>[2x]MSLKTVAVIGAMEQEIELLREMMENVKAVSFGRFSAYEGELAGKRMVLA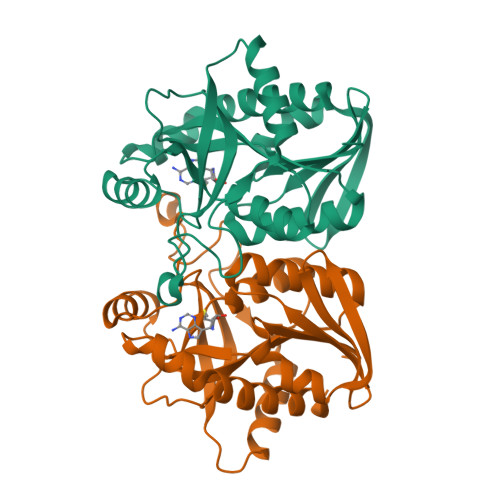LSGIGKVNAAVATAWIIREFAADCVINTGSAGGLGKGLKVGDVVIGTETAHHDVDVTAFGYAWGQVPQLPARFASDGILIEAAKRAARTFEGAAVEQGLIVSGDRFVHSSEGVAEIRKHFPEVKAVEMEAAAIAQTCHQLETPFVIIRAVSDSADEKADISFDEFLKTAAANSAKMVAEIVKSL> TAAGTACAACCACAGCATTCCAGAACACGTCAACAAATAAGGAACAAAACTCGTATT;> AAGCCAGAATGCCCTTTTAACTGAGGTTTAA;> TCATAACCCGTCGGATGTAGATG;> CAGAGGCCCATCAATATGAGTTTTTATA;> TTGTATCGGATTTTCATAGTTAGCGTAAACCCTCATAGGTGT;> GGAAGCAAACTCCATTGAGTTAAGCC;> TCAGATGATGGCAATTATCATATTTACAAAGTCTTTC;> GAGTAGATTTAGATAACCTGTTTA;> TTTTTGAGAGATATTTAGG;> CATCACGCAAATGCCGGAGAAGG;> ATATATCGGTTATGCGTGGGCGATGGTTGTTGTCATTGTCGGCGCAACTATCGGTATCAAGCTGTTTAAGAAATTCACCTCGAAAGCAAGCTGATAAACCGATACAATTAAAGGCTCCTTTTGGAGCCTTTTTTTTGGAGATTTTCAACGTGAAAAAATTATTATTCGCAATTCCTTTAGTTGTTCCTTTCTATTCTCACTCCGCTGAAACTGTTGAAAGTTGTTTAGCAAAATCCCATACAGAAAATTCATTTACTAACGTCTGGAAAGACGACAAAACTTTAGATCGTTACGCTAACTATGAGGGCTGTCTGTGGAATGCTACAGGCGTTGTAGTTTGTACTGGTGACGAAACTCAGTGTTACGGTACATGGGTTCCTATTGGGCTTGCTATCCCTGAAAATGAGGGTGGTGGCTCTGAGGGTGGCGGTTCTGAGGGTGGCGGTTCTGAGGGTGGCGGTACTAAACCTCCTGAGTACGGTGATACACCTATTCCGGGCTATACTTATATCAACCCTCTCGACGGCACTTATCCGCCTGGTACTGAGCAAAACCCCGCTAATCCTAATCCTTCTCTTGAGGAGTCTCAGCCTCTTAATACTTTCATGTTTCAGAATAATAGGTTCCGAAATAGGCAGGGGGCATTAACTGTTTATACGGGCACTGTTACTCAAGGCACTGACCCCGTTAAAACTTATTACCAGTACACTCCTGTATCATCAAAAGCCATGTATGACGCTTACTGGAACGGTAAATTCAGAGACTGCGCTTTCCATTCTGGCTTTAATGAGGATTTATTTGTTTGTGAATATCAAGGCCAATCGTCTGACCTGCCTCAACCTCCTGTCAATGCTGGCGGCGGCTCTGGTGGTGGTTCTGGTGGCGGCTCTGAGGGTGGTGGCTCTGAGGGTGGCGGTTCTGAGGGTGGCGGCTCTGAGGGAGGCGGTTCCGGTGGTGGCTCTGGTTCCGGTGATTTTGATTATGAAAAGATGGCAAACGCTAATAAGGGGGCTATGACCGAAAATGCCGATGAAAACGCGCTACAGTCTGACGCTAAAGGCAAACTTGATTCTGTCGCTACTGATTACGGTGCTGCTATCGATGGTTTCATTGGTGACGTTTCCGGCCTTGCTAATGGTAATGGTGCTACTGGTGATTTTGCTGGCTCTAATTCCCAAATGGCTCAAGTCGGTGACGGTGATAATTCACCTTTAATGAATAATTTCCGTCAATATTTACCTTCCCTCCCTCAATCGGTTGAATGTCGCCCTTTTGTCTTTGGCGCTGGTAAACCATATGAATTTTCTATTGATTGTGACAAAATAAACTTATTCCGTGGTGTCTTTGCGTTTCTTTTATATGTTGCCACCTTTATGTATGTATTTTCTACGTTTGCTAACATACTGCGTAATAAGGAGTCTTAATCATGCCAGTTCTTTTGGGTATTCCGTTATTATTGCGTTTCCTCGGTTTCCTTCTGGTAACTTTGTTCGGCTATCTGCTTACTTTTCTTAAAAAGGGCTTCGGTAAGATAGCTATTGCTATTTCATTGTTTCTTGCTCTTATTATTGGGCTTAACTCAATTCTTGTGGGTTATCTCTCTGATATTAGCGCTCAATTACCCTCTGACTTTGTTCAGGGTGTTCAGTTAATTCTCCCGTCTAATGCGCTTCCCTGTTTTTATGTTATTCTCTCTGTAAAGGCTGCTATTTTCATTTTTGACGTTAAACAAAAAATCGTTTCTTATTTGGATTGGGATAAATAATATGGCTGTTTATTTTGTAACTGGCAAATTAGGCTCTGGAAAGACGCTCGTTAGCGTTGGTAAGATTCAGGATAAAATTGTAGCTGGGTGCAAAATAGCAACTAATCTTGATTTAAGGCTTCAAAACCTCCCGCAAGTCGGGAGGTTCGCTAAAACGCCTCGCGTTCTTAGAATACCGGATAAGCCTTCTATATCTGATTTGCTTGCTATTGGGCGCGGTAATGATTCCTACGATGAAAATAAAAACGGCTTGCTTGTTCTCGATGAGTGCGGTACTTGGTTTAATACCCGTTCTTGGAATGATAAGGAAAGACAGCCGATTATTGATTGGTTTCTACATGCTCGTAAATTAGGATGGGATATTATTTTTCTTGTTCAGGACTTATCTATTGTTGATAAACAGGCGCGTTCTGCATTAGCTGAACATGTTGTTTATTGTCGTCGTCTGGACAGAATTACTTTACCTTTTGTCGGTACTTTATATTCTCTTATTACTGGCTCGAAAATGCCTCTGCCTAAATTACATGTTGGCGTTGTTAAATATGGCGATTCTCAATTAAGCCCTACTGTTGAGCGTTGGCTTTATACTGGTAAGAATTTGTATAACGCATATGATACTAAACAGGCTTTTTCTAGTAATTATGATTCCGGTGTTTATTCTTATTTAACGCCTTATTTATCACACGGTCGGTATTTCAAACCATTAAATTTAGGTCAGAAGATGAAATTAACTAAAATATATTTGAAAAAGTTTTCTCGCGTTCTTTGTCTTGCGATTGGATTTGCATCAGCATTTACATATAGTTATATAACCCAACCTAAGCCGGAGGTTAAAAAGGTAGTCTCTCAGACCTATGATTTTGATAAATTCACTATTGACTCTTCTCAGCGTCTTAATCTAAGCTATCGCTATGTTTTCAAGGATTCTAAGGGAAAATTAATTAATAGCGACGATTTACAGAAGCAAGGTTATTCACTCACATATATTGATTTATGTACTGTTTCCATTAAAAAAGGTAATTCAAATGAAATTGTTAAATGTAATTAATTTTGTTTTCTTGATGTTTGTTTCATCATCTTCTTTTGCTCAGGTAATTGAAATGAATAATTCGCCTCTGCGCGATTTTGTAACTTGGTATTCAAAGCAATCAGGCGAATCCGTTATTGTTTCTCCCGATGTAAAAGGTACTGTTACTGTATATTCATCTGACGTTAAACCTGAAAATCTACGCAATTTCTTTATTTCTGTTTTACGTGCAAATAATTTTGATATGGTAGGTTCTAACCCTTCCATTATTCAGAAGTATAATCCAAACAATCAGGATTATATTGATGAATTGCCATCATCTGATAATCAGGAATATGATGATAATTCCGCTCCTTCTGGTGGTTTCTTTGTTCCGCAAAATGATAATGTTACTCAAACTTTTAAAATTAATAACGTTCGGGCAAAGGATTTAATACGAGTTGTCGAATTGTTTGTAAAGTCTAATACTTCTAAATCCTCAAATGTATTATCTATTGACGGCTCTAATCTATTAGTTGTTAGTGCTCCTAAAGATATTTTAGATAACCTTCCTCAATTCCTTTCAACTGTTGATTTGCCAACTGACCAGATATTGATTGAGGGTTTGATATTTGAGGTTCAGCAAGGTGATGCTTTAGATTTTTCATTTGCTGCTGGCTCTCAGCGTGGCACTGTTGCAGGCGGTGTTAATACTGACCGCCTCACCTCTGTTTTATCTTCTGCTGGTGGTTCGTTCGGTATTTTTAATGGCGATGTTTTAGGGCTATCAGTTCGCGCATTAAAGACTAATAGCCATTCAAAAATATTGTCTGTGCCACGTATTCTTACGCTTTCAGGTCAGAAGGGTTCTATCTCTGTTGGCCAGAATGTCCCTTTTATTACTGGTCGTGTGACTGGTGAATCTGCCAATGTAAATAATCCATTTCAGACGATTGAGCGTCAAAATGTAGGTATTTCCATGAGCGTTTTTCCTGTTGCAATGGCTGGCGGTAATATTGTTCTGGATATTACCAGCAAGGCCGATAGTTTGAGTTCTTCTACTCAGGCAAGTGATGTTATTACTAATCAAAGAAGTATTGCTACAACGGTTAATTTGCGTGATGGACAGACTCTTTTACTCGGTGGCCTCACTGATTATAAAAACACTTCTCAGGATTCTGGCGTACCGTTCCTGTCTAAAATCCCTTTAATCGGCCTCCTGTTTAGCTCCCGCTCTGATTCTAACGAGGAAAGCACGTTATACGTGCTCGTCAAAGCAACCATAGTACGCGCCCTGTAGCGGCGCATTAAGCGCGGCGGGTGTGGTGGTTACGCGCAGCGTGACCGCTACACTTGCCAGCGCCCTAGCGCCCGCTCCTTTCGCTTTCTTCCCTTCCTTTCTCGCCACGTTCGCCGGCTTTCCCCGTCAAGCTCTAAATCGGGGGCTCCCTTTAGGGTTCCGATTTAGTGCTTTACGGCACCTCGACCCCAAAAAACTTGATTTGGGTGATGGTTCACGTAGTGGGCCATCGCCTGATAGACGGTTTTTCGCCCTTTGACGTTGGAGTCCACGTTCTTTAATAGTGGACTCTTGTTCCAAACTGGAACAACACTCAACCCTATCTCGGGCTATTCTTTTGATTTATAAGGGATTTTGCCGATTTCGGAACCACCATCAAACAGGATTTTCGCCTGCTGGGGCAAACCAGCGTGGACCGCTTGCTGCAACTCTCTCAGGGCCAGGCGGTGAAGGGCAATCAGCTGTTGCCCGTCTCACTGGTGAAAAGAAAAACCACCCTGGCGCCCAATACGCAAACCGCCTCTCCCCGCGCGTTGGCCGATTCATTAATGCAGCTGGCACGACAGGTTTCCCGACTGGAAAGCGGGCAGTGAGCGCAACGCAATTAATGTGAGTTAGCTCACTCATTAGGCACCCCAGGCTTTACACTTTATGCTTCCGGCTCGTATGTTGTGTGGAATTGTGAGCGGATAACAATTTCACACAGGAAACAGCTATGACCATGATTACGAATTCGAGCTCGGTACCCGGGGATCCTCTAGAGTCGACCTGCAGGCATGCAAGCTTGGCACTGGCCGTCGTTTTACAACGTCGTGACTGGGAAAACCCTGGCGTTACCCAACTTAATCGCCTTGCAGCACATCCCCCTTTCGCCAGCTGGCGTAATAGCGAAGAGGCCCGCACCGATCGCCCTTCCCAACAGTTGCGCAGCCTGAATGGCGAATGGCGCTTTGCCTGGTTTCCGGCACCAGAAGCGGTGCCGGAAAGCTGGCTGGAGTGCGATCTTCCTGAGGCCGATACTGTCGTCGTCCCCTCAAACTGGCAGATGCACGGTTACGATGCGCCCATCTACACCAACGTGACCTATCCCATTACGGTCAATCCGCCGTTTGTTCCCACGGAGAATCCGACGGGTTGTTACTCGCTCACATTTAATGTTGATGAAAGCTGGCTACAGGAAGGCCAGACGCGAATTATTTTTGATGGCGTTCCTATTGGTTAAAAAATGAGCTGATTTAACAAAAATTTAATGCGAATTTTAACAAAATATTAACGTTTACAATTTAAATATTTGCTTATACAATCTTCCTGTTTTTGGGGCTTTTCTGATTATCAACCGGGGTACATATGATTGACATGCTAGTTTTACGATTACCGTTCATCGATTCTCTTGTTTGCTCCAGACTCTCAGGCAATGACCTGATAGCCTTTGTAGATCTCTCAAAAATAGCTACCCTCTCCGGCATTAATTTATCAGCTAGAACGGTTGAATATCATATTGATGGTGATTTGACTGTCTCCGGCCTTTCTCACCCTTTTGAATCTTTACCTACACATTACTCAGGCATTGCATTTAAAATATATGAGGGTTCTAAAAATTTTTATCCTTGCGTTGAAATAAAGGCTTCTCCCGCAAAAGTATTACAGGGTCATAATGTTTTTGGTACAACCGATTTAGCTTTATGCTCTGAGGCTTTATTGCTTAATTTTGCTAATTCTTTGCCTTGCCTGTATGATTTATTGGATGTTAATGCTACTACTATTAGTAGAATTGATGCCACCTTTTCAGCTCGCGCCCCAAATGAAAATATAGCTAAACAGGTTATTGACCATTTGCGAAATGTATCTAATGGTCAAACTAAATCTACTCGTTCGCAGAATTGGGAATCAACTGTTATATGGAATGAAACTTCCAGACACCGTACTTTAGTTGCATATTTAAAACATGTTGAGCTACAGCATTATATTCAGCAATTAAGCTCTAAGCCATCCGCAAAAATGACCTCTTATCAAAAGGAGCAATTAAAGGTACTCTCTAATCCTGACCTGTTGGAGTTTGCTTCCGGTCTGGTTCGCTTTGAAGCTCGAATTAAAACGCGATATTTGAAGTCTTTCGGGCTTCCTCTTAATCTTTTTGATGCAATCCGCTTTGCTTCTGACTATAATAGTCAGGGTAAAGACCTGATTTTTGATTTATGGTCATTCTCGTTTTCTGAACTGTTTAAAGCATTTGAGGGGGATTCAATGAATATTTATGACGATTCCGCAGTATTGGACGCTATCCAGTCTAAACATTTTACTATTACCCCCTCTGGCAAAACTTCTTTTGCAAAAGCCTCTCGCTATTTTGGTTTTTATCGTCGTCTGGTAAACGAGGGTTATGATAGTGTTGCTCTTACTATGCCTCGTAATTCCTTTTGGCGTTATGTATCTGCATTAGTTGAATGTGGTATTCCTAAATCTCAACTGATGAATCTTTCTACCTGTAATAATGTTGTTCCGTTAGTTCGTTTTATTAACGTAGATTTTTCTTCCCAACGTCCTGACTGGTATAATGAGCCAGTTCTTAAAATCGCATAAGGTAATTCACAATGATTAAAGTTGAAATTAAACCATCTCAAGCCCAATTTACTACTCGTTCTGGTGTTTCTCGTCAGGGCAAGCCTTATTCACTGAATGAGCAGCTTTGTTACGTTGATTTGGGTAATGAATATCCGGTTCTTGTCAAGATTACTCTTGATGAAGGTCAGCCAGCCTATGCGCCTGGTCTGTACACCGTTCATCTGTCCTCTTTCAAAGTTGGTCAGTTCGGTTCCCTTATGATTGACCGTCTGCGCCTCGTTCCGGCTAAGTAACATGGAGCAGGTCGCGGATTTCGACACAATTTATCAGGCGATGATACAAATCTCCGTTGTACTTTGTTTCGCGCTTGGTATAATCGCTGGGGGTCAAAGATGAGTGTTTTAGTGTATTCTTTTGCCTCTTTCGTTTTAGGTTGGTGCCTTCGTAGTGGCATTACGTATTTTACCCGTTTAATGGAAACTTCCTCATGAAAAAGTCTTTAGTCCTCAAAGCCTCTGTAGCCGTTGCTACCCTCGTTCCGATGCTGTCTTTCGCTGCTGAGGGTGACGATCCCGCAAAAGCGGCCTTTAACTCCCTGCAAGCCTCAGCGACCGA;> GACAATATTTTTCGCGAG;> TAATCAGTAGCGACATAGTAAGAGCAAGGCTTTGTTTTGC;> GGGTCAGCGATTATAAAGAGGCAAAAGAAACGGCTATCGTCA;> AAACAAATACAGATAGCC;> AGATTAAGATTGGGTTAT;> ATTAATGCCGAGAGTCTG;> TCGCCCAGCAGGGAGACTTTTCAACATTGAAAGATTCA;> CAATAATTGTACAGGAGTAATCTT;> TTACGCCAGTTTCCCAGT;> TACTTTTCATCGTAGGAATCATTTAGT;> ATTGCCTGGAGAGGCCGTTCTGAGAAAGTAACCGTCACTTGCCTGAGTAGAAGA;> GTTCCGAAATCGGCAAATACTTCTTGATGGTG;> CGAGCCGGAAGCATAAAGGAAAGGACCTTGTAAAGCC;> ACGACGATAAAAGTAAAAT;> CCCGTATAAACTTCTTAAGATATTCAC;> GGCTGACCTAACAAAGCT;> ACCGTAATGGGAAGGGGACGA;> TTGAAAATAGAAACAGTACAAACTACAAATAGGAGATAAGTG;> AAGTAAGAATCCTCTGGCCTTACAGCTTCAGCGAAGGAACGAGGG;> AAGTTCTTAATTGTGTCTGGAAGTATTTTGCAC;> ATAGCAAGCATTTTGAAGGAACCAGCCGCCAGACAGGAGCAGTCTGGCTTTTGA;> GGTCCGATGAACGGTAATCGTAAAATT;> TATAATAAAAGAGTCTGTC;> TAGAACCCTTCTCGTAAGAATACGTGGCACA;> CAGAGGGTCACCAGATTTGTATCATC;> CTATTATCCCGGAAGAGCCACCACCCTCCAGCCCTGCTAAAC;> GACAAGAACAGCCGCCGC;> TGGTTCTCCGTTCAAATAAGATTAAGAGGAAGCC;> CGAATAATAATTAGGATTAGC;> GAGCGCTAGAAACAACTGGCACAAACGTAATAGTGCTTTTTAACCT;> TAAGTTGGGTAACGGACGGCC;> TATAGAAGGCTTATAACCTCCACCGCCTCTCAGAGAGACGATATTA;> CAACATGTACTACAAAGGCTAAGGAGGCCG;> ATCAGTGAGGCCACCGAGATCAA;> TGAGCTAACGTGCCAGCT;> CGTCACCAATGAAACCATAAGAATGCAACGATAGCAGCACCG;> TCAAGAGCCAGGCGACCCATGTACCGTAACACT;> CCAGCGGATATTCATTGTCATTTCTTAGAGTGAGTAACCGAAC;> GGCGCATTAATTAACAAAA;> TCGGTCGCTTAGTAAATTGGGCTGAATTAC;> TTAGACGAATAACACGCCACCCCCTCAGAGCCGCCAC;> GTTATTAATTGCGATGCAAGTTAA;> GCTATATTTTCATCTACTATTGCGCTTTTCCAG;> TTAATTGAGAATCGCCCGCTCAATGAATTAATTGACGAGTG;> GTTGAGTGTTGTTCCGCCA;> TCACATTTGGGGTGCCTAATGAG;> TAGCGTCCAATACTGAGCCAATTAGCGGAATCGTCATA;> CGAGATCCCCCTCAAACGAT;> CCACGCCTTTAGCCATATGGAGCGGAGACTTTACA;> CATCTGCAGGAAGAGCGAACCAGACC;> AAGCATCTTTAATCACCGCCTTAACAATTTTTCAATATATATCTTTAG;> GGAAGCGCAACAGTAACA;> AAATATCTAAACTGGTCAGGTCAGTATTA;> CTGCTCATCCGCAAAAAG;> GAGCAAACACGGTTGATA;> GAGAAGTTATTCAAGTAGCTAGTTTAGACTGGA;> AATTGCGATAGTAGTAGCA;> AGCAAAAGGTAATAACCAAAATAAAGTACAGCTAATGCAGAACGCGC;> TACTGGCGACAATCCGTAA;> CCTCAGAACTAAAAACAG;> TCTGTAAATCGTCGCTATCGTAACCGTG;> CCCTCAGGATACCGAGTAACAGTG;> GAGAGTACCTTTAATTGCTATAATGCATGTGCT;> AACAACTAACATATCAAACAACAGTGCCA;> GTGGAGGCAAAGACGTTGGGAAG;> CTTACTTGAGCCATTTGGG;> CGGTACAGTTTGGAACAAG;> TCGGGAACAACGCGTCGGTTGTACCA;> CATTAAAGGCAGTAGGGC;> TGATACAGGGAAATTATT;> GCTCATTCAGATTCCCGCAACTATCGACTCAGTGCCAAGCTTGCATAAAGG;> CCTTGCTTTAGAATCCTTGAAAAGAGTCAGAAAATCGCAAAG;> ACGTTGGTGAATAGTTAATGCCCCCTTACTCAGCCCTCAG;> ATAAGAGACCCAAAAGGCTTGCCCTGACGAGAAAC;> ACATTTGAGGATTTAGGCCG;> TTAAACCAAGTACGAGAACAA;> ATATCATATGGCTGCGCACGGGGAAAGCCGG;> ATTAAAGGGATTTTAGACAGGAAGAATCCT;> CTGGCCACCCGCCACTGACAGAGA;> AATATTCATTGAGCGCAGACGGTC;> AATCATAAGGGAGCATAGGCT;> ACATCAATCATACAGAACGAGGAGGCTTCGCATAAGTGTCGACTGCTCC;> AGTACATAAACATCAAGACGCAATTACCGAAGGAAAGCGGTT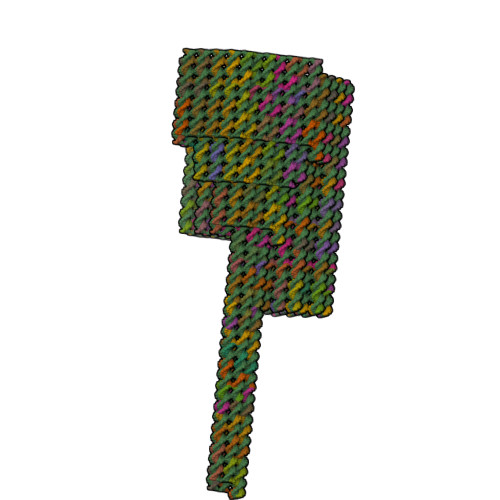GAGCGCCGACTTGCGGG;> AACTTTCAAAGGAGCATGAAAGTATTAAAGAGGGTGGGATAG;> TTGCGTTTTGTTTACACCA;> CACGACGTTGTAAAACCCAGGGTCTGGCGA;> TTAACATCCAATAAATCATAGCTAAACGGGGAGCGTATTG;> TACAAACTAGCATGTCGCTGGCAGGCGAGA;> AGTCCACTATTAAAATCAG;> GCATTAATGAATCGGCACCTGTC;> TGAGGATGTTACCTTTGAAAGAGGAGTAAGCGT;> ACCGAACGGATTGCATCAAAATCGCGTT;> GAGCCACCACCGGACGACTTGCAACGCTCCTCAAAACTAATA;> ATTTGAATTACCTTTTTACATTTTACCAGA;> ACAGAGGCTTTGAGTAAAACGACCAAGCGGCCGGAAA;> CCCAATCAAATGAAGAACAAAGCTATCTAATAACGTAAAGGTGG;> AATTGAGGAAGGTTCCTTTGCCATTATCTGGAAGGGTAAAACTTACAAACCTGAGC;> AGCATAAACAGGCACATCAATTTTGGGGGAATGGCTAATGCGCGAACTGATAGC;> TACTAGAAACGCCGCGCT;> TTAGAGAACGTGGACTCCA;> GGCGCCAAACAGCTTATATTTTAAAT;> GAGGGAAAAGGGCGTTAAATATACCGACTGCCGTAAAG;> CATACATCTGAATTAGCAATAGTCAGAGAAGAAATATACTTCTGA;> ATTAGCGTTTGCGCCGCTTAATGACATTTAACG;> CGACAGTATCGGAAACCA;> TAGCATACACTTCTTTGACCCCCAGTGCCTTGATAGTTGGCAGGTCCCA;> ATTTGCCAGTCCTGATTA;> GAGCATTCGACAGAAACCTTGGATTTGCGTAGCTGATTGCTTT;> TCAGTGCGGGATACCACATTCAA;> ATCAGAAAATATTTTGCTACGTGAAC;> ACGTGCTCTAGGGCAATCATAAAACAGGTTCAGAATTTACCCTGACTATTA;> ATAAAAGGTTTGAGGCGGGACATT;> CAACTGCTTTAAACAGAAGATTG;> TGAACGGAAGAGCAAATATCATTTGCACGTTAGAACCTACCATAGTTGGGAAGGGC;> CAACTTTAAATGGTCATTTGACCCCATTAACGAACCACCAGCAGAAGATAAAACAG;> CCAGCTTATTCATTGACTC;> GTCGTCTTTGCATCAGACACCAG;> TGTTTTAAATATAATTCTGCGAAC;> GATTAGAAAGTATTAATTATCCATCAATCGTCAGAGAGAAACAATTAATTTAATGGAAAC;> TCCAAGATTAAGCAAAAACGGGTA;> TATAAAATAAGGCGACATT;> TGGTTGCTTTCGGTCACCGTTA;> CACCAGTGAAAGCGGTCC;> TGGTTTACCAATCATAAT;> CTTATGCGATTTTAAGGGCAT;> AAAAGAACAAAAGAATGAAATTACCGTTCCACAGA;> CCACAGAATTTTCATGATATAAGTATAGTCTGAAACCTTTAA;> CCAGCTAATCAAGATACCGCGCCCA;> TCAATCACCTCAGCAGCAAATGAAAA;> AAAACATTATGACCCTGTAATACTTT;> GATAGCAAATATTTAATCAAGTT;> TAATGCGCCGCTACAGCCACACCAAGCCTGACACCGGAGCGCCA;> GACGGGCGGGTGGTTTTTCTTTT;> AATCAAAAATTCGCGTTAAATCAGCTCATTACGTTAAGCCCCAATGTACCCAGAGAAT;> CAGTCAGGAATTAGCAATAAAGCC;> AGAGGCGAACAGCTTTCCGGCACCGCTTCCATTCA;> GAGTTTCGTCACGGAACAACTAAAGGAATTG;> TGCTTTCATTCCATATAACAGTTGTGAATATCAACGTTCATCAAACCAGGC;> TAGAGGATCCCCGGGTACCGAGC;> AGAACCCTCAGATTGCCTGGC;> TGGGTTAATTTGTAAATGCTTAGGCGCTGAGAACATAGATGTGAGTGAATAA;> ACGTCAAAGGGCGAAAGGA;> CCTGAGAGAGATTATTTTTTGACGCGCCAGCCTGGTAA;> TAGTCAGAAGTTGGAATAAG;> TCATCAACTGGCTCAACGGAATCATGAGGCCACTAAACGGAGTAGCACCCACCGACCAGT;> GAATACCAAGAGAAATAGGTAATT;> GGGTAAAATCATAACCCATAACGAATAGATACCAATCAATAATCGGCTG;> TTTAGCGCCGGTATTCTAAGAAC;> GCAGGAAGTACGGCTGAATCCTTTTGAACCCACAAGAAACAGGTCAGGATTA;> AAATTGTAGAAAAGTCCTACATGTTCCGACAAACAGTCAAATCAATTTTCGAGCCAGT;> GACCTAAATAACCCTAAA;> AGCGAAAAACCGTCTATCA;> TCACACGCCGCCCTTCAACCAGTA;> CAATAGAAAAGAAAACATACAGAATACCGATGATGAAACAAATCAATATCGATAGCTT;> TGTAGCGCGTTTTTTCGGTCATAGCCCCCTT;> ACGGATTCGCATTTTCAACACCCTAATAGCACCTCAGA;> CCGCCAGAGGTTTAGTAC;> GCGAGGCGTCAGAGCCTA;> ATCTAAAGCATAGATAAT;> TCTTTCCTCAACTTATTTTATCAT;> TTAAATTTTTGTCTGGCCTTCCTG;> AAGGAAGACCCAAAATTGTAATTTTAACCAATAACGCG;> ACGCTGGCTGAAATGGTTGCAGC;> CAAAGCTGACCAATTAGCCGGAA;> AAAAATCTACGTTAATAAA;> GTACCTTTTACATCGGTGAATAT;> AACCGCCCGATCTAGAATTTTCTGTATGGGTTTATTCGGAAC;> TCGAATTCGTAATCATGGCCGAA;> GCAATGCCCATCATATCCTGAGTA;> AGAAAACTTTTAATCGCAAGACTACAATTTATTTTTCCC;> CGAACGTAGTGTAGGACGAGCACGTATA;> CTCATGGAAATAACGAGCATTTT;> ACACCACTATTTTGCAAATCCTCAAATATAT;> TTAGGAAGAAGCCTGCAAGGATAA;> GGCAAAGCGTCTTCGCTA;> CAAGCCCACGCCTGTCAGCGGAGTGAGAATCTCCAAGACTCC;> AGGTGAGGCGTTGGCAAATCAACAGTTGGCCT;> AAAAATACTAATTTCCTACATACATTGGCAGATTCACCAG;> TTTATTTGAAAAGAATAATTTAGTAAAGCCAAATATTTAACAACGC;> GGGAGCCCCCGATTTAAAATCGGTTAA;> CAGCAGGCAATATTACCTCAATCGTTTTGCCC;> CAACATATAAAATTCATA;> TCAGGAATTACGAGGCAGAATCAAGTTTGC;> GGCTGCGCAACTTCAAAATTAGAGAGAT;> AAAGTACCGAAGGCACCAACCGACTAAAGTTA;> ACACCGCCTGCCCTCAAATCCTGA;> CTGTTTATCAACCCAAAAGTTGAGATACGAACTATTATAC;> AAGAGGAACGCCATCATGAGCGA;> GGCGATGGCCCATTAAAATTCGCA;> CATTGCAACAGGAAAAACG;> CGAAAGACTGGGAACAATCAACATTA;> CTTTAGCAGGTAATTACGTCAGAC;> GCGGGCCCCATTCGCTGGTGCCGGCCTCCAGTTTGTAGGTCACGT;> CGCCACTCAAAAACACCCTCAGAA;> CGCTGAGAGCTGCTGAAAACGAGCATAAACACAGAGAGGGAGAATTTAAGAAAGGA;> ATGTGTACAGACCTGTCGGTAAAG;> ATAACTATATCATCTTCT;> CATCGGAAGAAGCGGGCGTTCCTCGAGCGGGAGCTAAACTCA;> ACTCAAACTATCATAAACAGAACAAG;> TTAATTTACGCAGTATGTTAGTGATTAATCAATTAATCGCGC;> CTAATGCAGATACTCGTTTACCAG;> GATCGGTAAGGGGGTGTAGCTCAACA;> ATCACCGGCCTATTCAGCTTGCTTTCGAAGTAAATAAGTTTT;> AAATATCATAGCTGTTTCCTGTG;> TAAAGTAATTGACGACAGGCCTTG;> TAGCCAGCTTTCAACGGCGGATTG;> TTTTGGGGTCGAGGCGTGT;> CCTGTTTTGATTAGTATATCCAGAACGAAAAT;> CTTATCGAGCTTCAAATCGCACT;> CTATACGTAATGAAGTTTCCATTAAAC;> ATAAATTTTGCGAAACGATTGATGG;> CCGTCGGAGGCTGAAAAAAAGGCTCCAAACAGTTTAGCATT;> CCTAAAACATCGATTAGA;> AATAAGAGAATATAGCGAGACA;> AATGAAAATAATCAGGTCAACGAGAATGACCATA;> CACTGAGCTTGGTAACCAGGCGCGTACTA;> ATAACATTGTAGCAAATCCCTAAGAATAGCCCGAGATAGG;> AACCGAGGAAAAAACAAAATA;> ATAATCCTGATTGTACCAGAATATTTATATCTTACCGGGAGGAATCAGA;> GGGGTTTTGCTCAGTAAAGGATTTTTTCACG;> TGAAATTGTTATCCGCTCGTCTT;> ATTCAAAAGGGTAGCTGATAA;> GTAACAGGTCTGAGAGACA;> GAACAAAGTAACAATTTC;> GCCTGATAAATTCCGATATAT;> TATTAACAATTCCACACAACATA;> CCGGCTGATGTCACAATAAGACAAGGTAAATTCACCGTATTACCATTAGCAAGCGAAAC> MVSSKKFNQVDKGRGMISENYIEPAFLLPDLIEIQRSSFR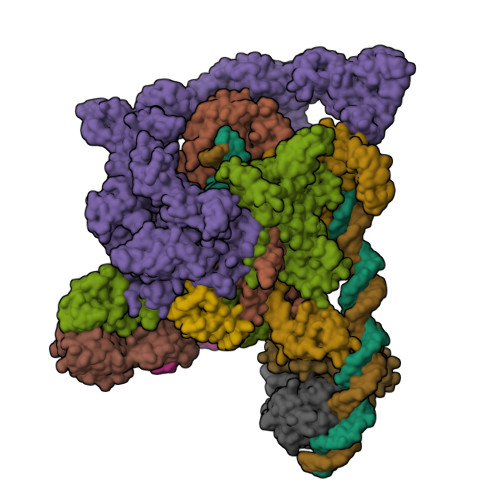WFLEEGLIEELNSFSPITDYTGKLELHFLGHNYKLKEPKYSVEEAKRRDSTYAVQMYVPTRLLNKETGDIKEQEVFIGDLPLMTDRGTFIINGAERVIVNQIVRSPGVYYKSEIDKNGRRTYSASLIPNRGAWLKFETDRNDLVWVRIDKTRKLSAQVLLKALGLSDNEIFDALRHPEYFQKTIEKEGQFSEEEALMELYRKLRPGEPPTVLGGQQLLDSRFFDPKRYDLGRVGRYKLNKKLRLSVPDTVRVLTSGDILAAVDYLINLEYDIGSIDDIDHLGNRRVRSVGELLQNQVRVGLNRLERIIRERMTVSDAEVLTPASLVNPKPLVAAIKEFFGSSQLSQFMDQTNPLAELTHKRRLSALGPGGLTRERAGFAVRDIHPSHYGRICPIETPEGPNAGLIGSLATHARVNQYGFLETPFRPVENGRVRFDQPAAYMTADEEDDLRVAPGDIPVDENGYIIGPQVPVRYRQEFSTTTPEQVDYVAVSPVQIVSVATSMIPFLEHDDANRALMGSNMQRQAVPLLKPERPLVGTGLEAQGARDSGMVIVSRTDGDVVYVDATEIRVRVSGQLPTASGKSTDNGQLTSQKGQEIRYTVSKYQRSNQDTCLNQKPLVRIGERVVAGQVLADGSSTEGGELALGQNIVVAYMPWEGYNYEDAILISERLVQDDIYTSIHIEKYEIEARQTKLGPEEITREIPNVGEDALRQLDEQGIIRIGAWVEAGDILVGKVTPKGESDQPPEEKLLRAIFGEKARDVRDNSLRVPNGEKGRVVDVRLFTREQGDELPPGANMVVRVYVAQKRKIQVGDKMAGRHGNKGIISRILPIEDMPYLPDGSPVDIVLNPLGVPSRMNVGQVFECLLGWAGHTLGVRFKITPFDEMYGEESSRRIVHGKLQEARDETGKDWVYNPDDPGKIMVYDGRTGEAFDRPVTIGVAYMLKLVHLVDDKIHARSTGPYSLVTQQPLGGKAQQGGQRFGEMEVWALEAFGAAYTLQELLTVKSDDMQGRNEALNAIVKGKAIPRPGTPESFKVLMRELQSLGLDIAVHKVETQADGSSLDVEVDLMADQLARRTPPRPTYESLSRESLDDDE;> MIFRNRVVDKGQLRNLISWAFTHYGTARTAVMADKLKDLGFRYATRAGVSISVDDLMVPPSKRSLLEAAEEEIRATEVRYQRGEITEVERFQKVIDTWNGTSEALKDEVVTHFKQTNPLNSVYMMAFSGARGNISQVRQLVGMRGLMADPQGEIIDLPIKTNFREGLTVTEYIISSYGARKGLVDTALRTADSGYLTRRLVDVSQDVIIREIDCGTTRGIPVRPMTEGSKTLIKLSTRLLGRVVGEDVIHPKTKEVIAPRNTPISDDLAKEIEKAGVAEVVVRSPLTCEAARSVCQHCYGWSLAHAKMVDLGEAVGIIAAQSIGEPGTQLTMRTFHTGGVFTGEVAQQVRSKMDGTIKLPRKLRTRTHRTRHGEDALFVESNGIMILEPRKEGSETPAPQEIHVTQGSTIYIVDGQQVKKGQLLAEVALGGRTTRTNTEKAVKDVASDLAGEVKFAEVVPEQKTDRQGNTTTTAARGGLIWILSGEVYNLPPGAELVVKNGDRVETNGVLAETKLTTIHGGVVRLPEATPGKSTREIEIITASVVLDQATVTVQSSQGRNNYLITTGNNQVFNLRATPGTKVQNGQVVAELIDDRYRTTTGGFLKFAGVEVQKKGKAKLGYEVVQGGTLLWIPEETHEVNKDISLLLVEDGQYVEAGTEVVKDIFCQNSGVVEVTQKNDILREVVVKPGELLMVDDPEAVIGRDNTLLQPGEELLGQVATELRYIQYVESPEGPALLSRPVVEFAVPSNPDVPSTTSVSQQTGRSIQMRAVQRLPYKDSERVKSVEGVELLRTQLVLEIEQEGEQEHNASPLAADIELIPDLEDADVQRLQLVILESLVLRRDIAADATQGSTQTSLEVKDGDTIVPGSVVARTQILSKEGGIVRGVQKGSEAVRRCLVLRHSDMATLNISAKPKVKAGDLIVAGTELAPGIFAEESGQIVGVKNAGESTTTQDAALSTQNYAVTIRAGRPYRVSPGAVLQIEDGDLVQRGDNLVLLVFERAKTGDIIQGLPRIEELLEARKPKEACILAKRGGEVKVVYGDGDEAIAIKVIESNGVVTDYPLGPGQNLAMPDGSVVPAGQPLSDGPSNPHEILEVFFSLGSEDGVYACASHALQKVQTFLVNEVQMVYQSQGIDIADKHIEVIVRQMTNKVRIDDGGDTTMLPGELVELRQVEQVNEAMAITGGARAQYTPVLLGITKASLNTDSFISAASFQETTRVLTEAAIEGKSDWLRGLKENVIIGRLIPAGTGYNTYDEPGMLEDYSTLETTSVLDETDDPLDMVLDDRTARAYNLDSPGLAETGFNNRRSILDDDELIADEIHDLVEAEVEVDDEVDDDYEDDDEDDDDYED;>[2x]MVAQFQIECVESNTEESRNHYSKFILEPLERGQGTTVGNALRRVLLSNLEGTAVTAVRIAGVSHEFATVPGVREDVLEIIMRMKEVILKSYSSQAQIGRLLVNGPTTITASHFDLPSEVEVIDPTQYVATIAEGGKLEMEFRIERGKGYRTVERGREEATSLDFLQIDSIFMPVRKVNYSVEEVRADGSIPKDRLLLEVWTNGSISPQEALSSAAGILVDLFNPLKDISLEPTDTN;> MRPAQTNQFDYVKIGLASPERIRQWGERTLPNGQVVGEVTKPETINYRTLKPEMDGLFCERIFGPAKDWECHCGKYKRVRHRGIVCERCGVEVTESRVRRHRMGYIKLAAPVAHVWYLKGIPSYISILLDMPLRDVEQIVYFNSYVVLSPGNAETLTYKQLLSEDQWLEIEDQIYSEDSQLQGVEVGIGAEALLRLLADINLEQEAESLREEIGSAKGQKRAKLIKRLRVIDNFIATGSKPEWMVMTVIPVIPPDLRPMVQLDGGRFATSDLNDLYRRVINRNNRLARLQEILAPEIIVRNEKRMLQEAVDALIDNGRRGRTVVGANNRPLKSLSDIIEGKQGRFRQNLLGKRVDYSGRSVIVVGPKLKIHQCGLPREMAIELFQPFVINRLIRSGMVNNIKAAKKLISRNDPSVWDVLEEVIEGHPVMLNRAPTLHRLGIQAFEPILVEGRAIQLHPLVCPAFNADFDGDQMAVHVPLSLESQAEARLLMLASNNILSPATGRPIITPSQDMVLGAYYLTAENPGATKGAGKYFASLDDVIMAFQQEQIDLHAYVYVRFDGDVESDQPDTEPVKVTTNEDGSRTVLYKYRRVREDAQGNVISQYIYTTPGRVIYNKAIQEALAS;> MLKRSKFETTQSQIMHRAEDLISAASNRYRITVQVANRAKRRRYEEFESAEDAMMKPVLRAIIEMSDELTQPEIIGEI;> MNQANNVLDSIYQPDLEIMNQPEIELDDLLIEEDEDLLLADDGDIDEFLEPQTDEDDAKSGKAAKSRRRTQSKKKHYTEDSIRLYLQEIGRIRLLRADEEIELARKIADLLELERVRERLSEKLERDPRDSEWAEAVQLPLPAFRYRLHIGRRAKDKMVQSNLRLVVSIAKKYMNRGLSFQDLIQEGSLGLIRAAEKFDHEKGYKFSTYATWWIRQAITRAIADQSRTIRLPVHLYETISRIKKTTKLLSQEMGRKPTEEEIATRMEMTIEKLRFIAKSAQLPISLETPIGKEEDSRLGDFIESDGETPEDQVSKNLLREDLEKVLDSLSPRERDVLRLRYGLDDGRMKTLEEIGQIFNVTRERIRQIEAKALRKLRHPNRNSVLKEYIR;>[2x]MIVTQDKALANVFRQMATGAFPPVVETFERNKTIFFPGDPAERVYFLLKGAVKLSRVYEAGEEITVALLRENSVFGVLSLLTGNKSDRFYHAVAFTPVELLSAPIEQVEQALKENPELSMLMLRGLSSRILQTEMMIETLAHRDMGSRLVSFLLILCRDFGVPCADGITIDLKLSHQAIAEAIGSTRVTVTRLLGDLREKKMISIHKKKITVHKPVTLSRQFT> MATV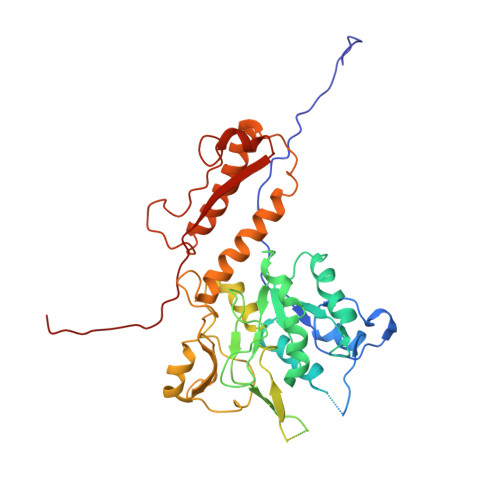TSVPGVYIEEDASPAMSVSASATAVPLFVARFTPLKPELAGVITRIGSWLDYTILFDSNVPSSARVTVSSTAVEPSPEFDALETASSKATTTYTYQIDDTEVVDPTASVALRLYFQNGGGPCYLYPLEKADDNGPLAALPDLIDEVGEITLLASPDPDETYRTAVYGALAASLDQHKGYFLLADSVNGDAPSAVGGSAQVAVYYPNVEVPHTRKLDDAEVAIDGYLDDEGKAVTTLAALRVVNTEFAGEIAQSLSGDLSAPLSLPPSALIAGVYGKTDGERGVWKAPANVVLNGVSDVSVRVTNEQQAELNPKGINVIRHFSDRGLVVWGSRTQKDDDDWRYIPVRRLFDAAERDIKKALQPMVFEPNSQLTWKRVQTAIDNYLYRLWQQGALAGNKAEEAYFVRVGKGITMTQDEINQGKMIIQVGMAAVRPAEFIILKFTQDMSQ>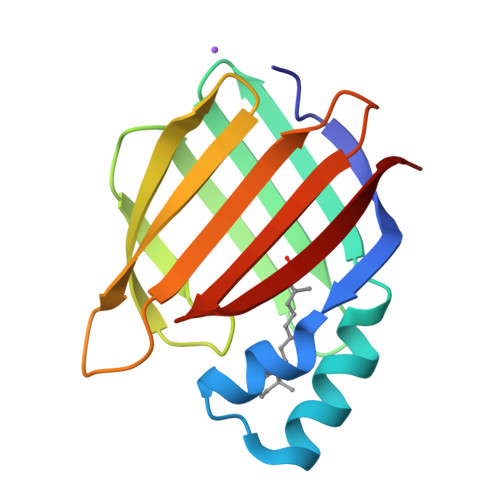 PNFSGNWKIIRSENFEELLKVLGVNVMLRKIAVAAASKPAVEIKQEGDTFYIKTSTTVRTTEINFKVGEEFEEQTVDGRPCKSLVKWESENKMVCEQKLLKGEGPKTSWTRELTNDGELILTMTADDVVCTKVFVRE>MIGTQIVTERLVALLESGTEKVLLIDSRPFVEYNTSHILEAININCSKLMKRRLQQDKVLITELIQHSAKHKVDIDCSQ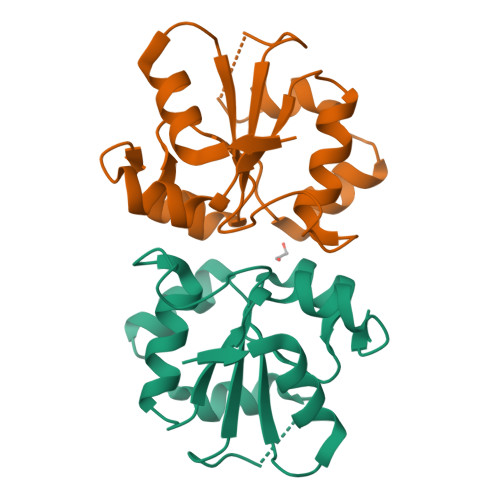KVVVYDQSSQDVASLSSDCFLTVLLGKLEKSFNSVHLLAGGFAEFSRCFPGLCEGLEHHHHHH[4x]> MIRTYPPVSFFFEVVFQGENLDKDVVETRFQSVTGLSVDMQTETL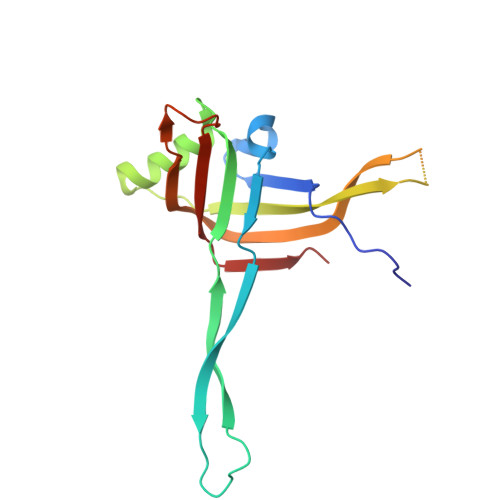KEGGENRFEHILPVRTKYDPLVLKRGLVNDSQMVKWCMDAILNFDIRPMNLLVRLLHIERSDPNQPPEAIATGGSSTIAPLMTWKVINAWPKKWSVSEFNAEQNSIAVESLELNYSYFETLK> MLTRFRSAVLRGAVSITGARAASTAPVADHKGRVGHVSQVIGAVVDVHFADGVPPVLTALDVVDKLGRDEPLTLEIVQHLDAHTGRCIAMQTTDLLKLKAKVVSTGGNISVPVGRETLGRIFNVLGDAIDQRGPVGEKLRMPIHAVAPKLADQAAEDAVLTTGIKVIDLILPYCKGGKIGLFGGAGVGKTVIIMELINNVAKGHGGFSVFAGVGERTREGTDLYLEMMQSKVIDLKGESKCVLVYGQMNEPPGARARVAQSALTMAEYFRDVEGQDVLLFIDNIFR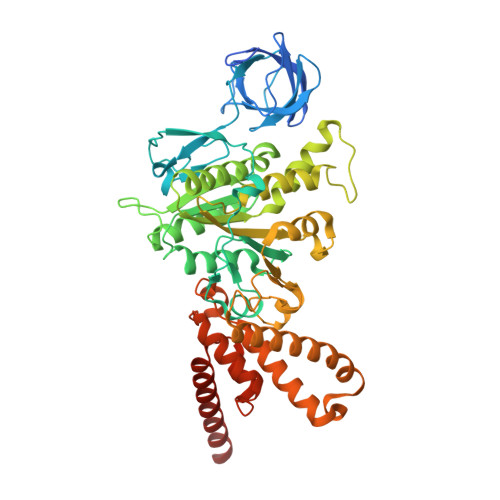FTQANSEVSALLGRIPAAVGYQPTLAEDLGQLQERITSTTKGSITSVQAVYVPADDITDPAPATTFSHLDATTVLDRAVAESGIYPAVNPLECASRIMDPDVISVDHYNVAQDVVQMLTKYRELQDIIAVLGIDELSEEDKLIVDRARKLVKFLSQPFQVAEVFTGMTGHYVQLDDTIDSFSGLLMGTYDQVPEMAFYMVGGINSVLEKAKKMAEEAAELEKMRRARVAQASS> NTGLLESQLSRHDQMLSVHDIRLADMDLRFQVLETASYNGVLIWKIRDYKRRKQEAVMGKTLSLYSQPFYTGYFGYKMCARVYLNGDGMGKGTHLSLFFVIMRGEYDALLPWPFKQKVTLMLMDQGSSRRHLGDAFKPDPNSSSFKKPTGEMNIASGCPVFVAQTV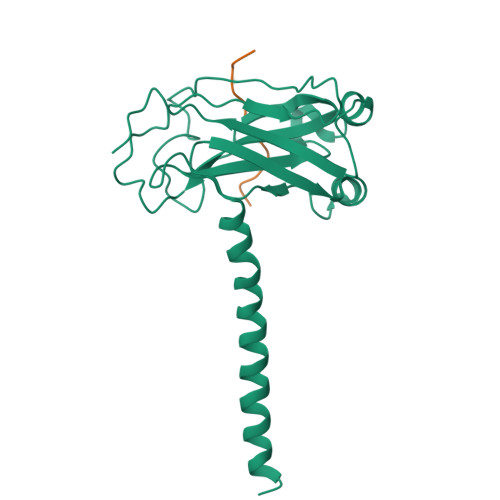LENGTYIKDDTIFIKVIVDTSDLPDP;> CSVPIQCTDKT> QPSCRQEEFLVGDECCPMCNPGYHVKQVCSEHTGTVCAPCPPQTYTAHANGLSKCLPCGVCDPDMGLLTWQECSSWKDTVCRCIPGYFCENQDGSHCSTCLQHTTGHHH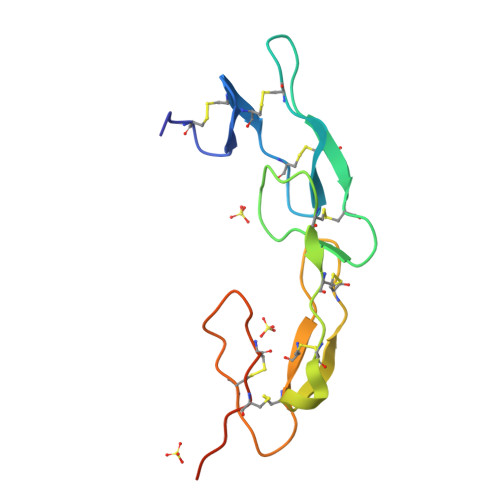HHH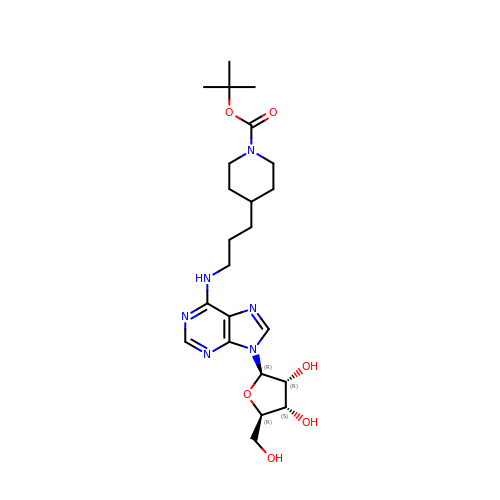N-{3-[1-(tert-butoxycarbonyl)piperidin-4-yl]propyl}adenosine | C23 H36 N6 O6 | NYCVBKCHESHFLR-QTQZEZTPSA-N METHYL 5,7-DIHYDROXY-2-METHYL-4,6,11-TRIOXO-3,4,6,11-TETRAHYDROTETRACENE-1-CARBOXYLATE | C21 H14 O7 | 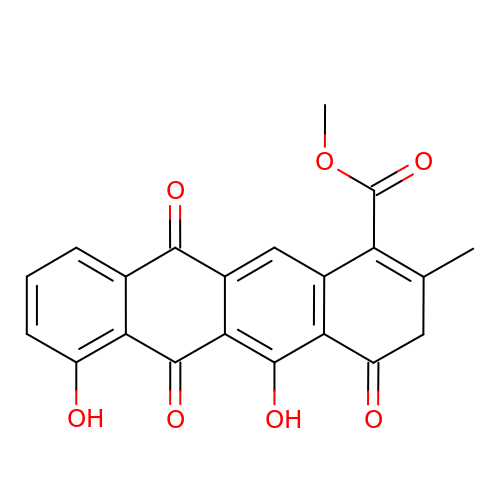QHNJNOBWURJIEK-UHFFFAOYSA-N>[4x]GAGSMKKLLNTLYVTQPDTYLSLDGDNVVLLKEQEKLGRLPLHNLEAIVGFGYTGASPALMGYCAERNISITFLTKNGRFLARVVGESRGNVVLRKTQYRISENDQESTKIARNFITGKVYNSKWMLERMTREHPLRVNVEQFKATSQLLSVMMQEIRNCDSLESLRGWEGQAAINYNKVFDQMILQQKEEFAFHGRSRRPPKDNVNAMLSFAYTLLANDVAAALETVGLDAYVGFMHQDRPGRASLALDLMEELRGLYADRFVLSLINRKEMTADGFYKKENGAVLMTDEARKTFLKAWQTKKQEKITHPYLGEKMSWGLVPYVQALLLARFLRGDLDEYPPFLWK;>[2x]GAGSMLVLITYDVQTSSMGGTKRLRKV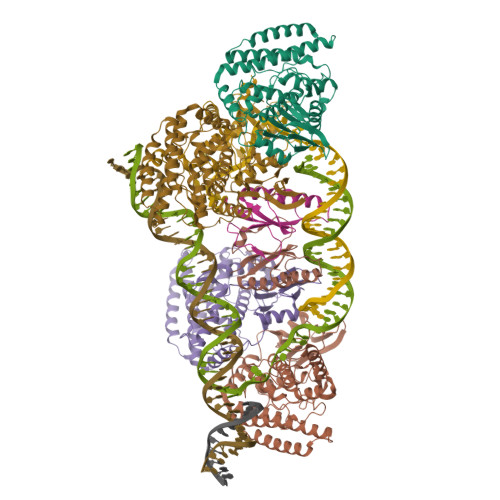AKACQNYGQRVQNSVFECIVDSTQLTSLKLELTSLIDEEKDSLRIYRLGNNYKTKVEHIGAKPSIDLEDPLIF;> ASNEEDRYLMLSGLQHFQFCKRQWALIHIEQQWEENVRTIEGQHLHKKADQPFMKEKRGSKLTVRAMPIQSKNLQISGICDVVEFVQDSEGIELSGVSGSYKAFPVEYKRGKPKKGDEDIVQLVAQAMCLEEMLVCRIDKGYLFYNEIKHRVEVPITDALRDKVVQMAKEMHHYYENRHTPKVKTGPFCNNCSLQSICLPKLMNKRSVKRYIEGRLSE>MRSYDMNVETAAELSAVNDILASIGEPPVSTLEGDANADAANARRILNKINRQIQSRGWTFNIEEGITLLPDVYSNLIVYSDDYLSLMSTSGQSIYVNRGGYVYDRTSQS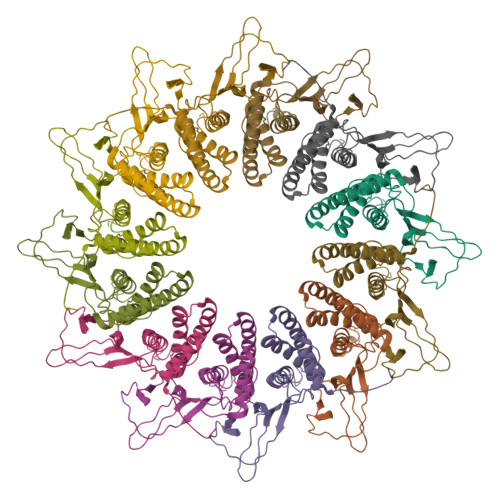DRFDSGITVNIIRLRDYDEMPECFRYWIVTKASRQFNNRFFGAPEVEGVLQEEEDEARRLCMEYEMDYGGYNMLDGDAFTSGLLTR[12x]> GSMGPRNDKIKHVQNQVDEVIDVMQENITKVIERGERLDELQDKSESLSDNATAFSNRSKQLRRQMWWRGCKIK;> GSMRETAIQQLEADILDVNQIFKDLAMMIHDQGDLIDSIEANVESSEVHVERASDQLQRAAYYQKKSRKKM;> GSMRAHLLDNTERLERSSRRLEAGYQIAVETEQIGQEMLENLSHDRERIQRARERLRETDANLGKSSRILTGMLRRIIQNR;> GSHMASMTGGNNMGRMQDEQLELVSGSIGVLKNMSQRIGGELEEQAVMLE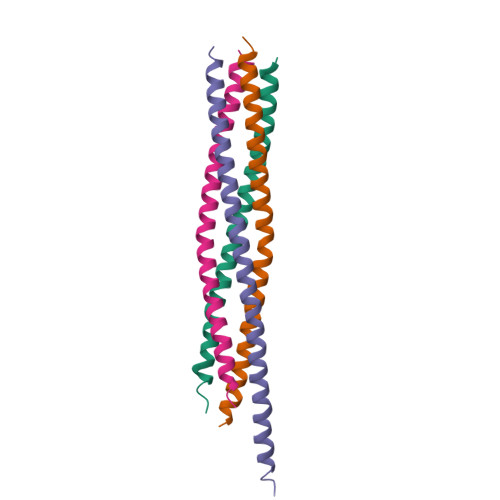DFSHELESTQSRLDNVMKKLAKVSHMTSDRRQ> MRGSHHHHHHTDPQGDAAQKTDTSHHDQDHPTFNKITPNLAEFAFSLYRQLAHQSNSTNIFFSPVSIATAFAMLSLGTKADTHDEILEGLNFNLTEIPEAQIHEGFQELLRTLNQPDSQLQLTFGNGLFLSEGLKLVDKFLEDVKKLYHSEAFTVNFGDTEEAKKQINDYVEKGTQGKIVDLVKELDRDTVFALVNYIFFKGKWERPFEVKDTEEEDFHVDQVTTVKVPMMKRLGMFNIQHCKKLSSWVLLMKYLGNATAIFFLPDEGKLQHLENELTHDIITKFLENEDRRSASLHLPKLSITGTYDLKSVLGQLGITKVFSNGADLSGVTEEAPLKLSKAVHKAVLTIDEKGTEAAGAMFLEAIPMSIPPEVKFNKPFVFLMIEQNTKSPLFMGKVVNPTQK

The plasma protein α1-antitrypsin is principally synthesised by hepatocytes and protects lung tissue from degradation by inhibiting neutrophil elastase. It is the archetypal member of the serpin (serine protease inhibitor) superfamily of proteins. In common with other inhibitory serpins, the native fold of α1-antitrypsin is metastable and this property is utilised in the characteristic serpin mechanism of action.

The 2.2 Å crystal structure of Thr114Phe α1-antitrypsin adopts the classic structure of a serpin fold in the native conformation. The polypeptide chain spanning residues 24–393 is highly ordered with the exception of residues 344–351. The root-mean-square deviation (r.m.s.d.) of the mutant and wild-type structures, based on Cα positions, is 0.4 Å. The lack of perturbation elsewhere in the overall structure of Thr114Phe α1-antitrypsin implies that the mutation must be mediating its effect on the fold stability of native α1-antitrypsin from within the cavity flanking β-sheet A. The cavity is well defined in this high-resolution structure, permitting interpretation of the effect of the mutation on cavity filling at the side-chain level. Phe114 makes no interactions with nearby residues, and therefore, its effects are entirely due to partial filling of the cavity and changes in its packing environment during unfolding and polymerisation. The aromatic group of Phe114 closes the upper part of the cavity with its side chain just 3.7 Å from Leu103 and 4.0 Å from Asn104 at the top of helix D, distances that permit favourable van der Waals contacts. The volume partially filling the cavity in Thr114Phe α1-antitrypsin is in a region of high-solvent accessibility in the wild-type protein and also yields the therapeutically desirable combination of effective blockade of polymerisation whilst maintaining inhibitory function. The estimated size of this ideal pharmacophore is 59 Å3, equivalent to 22% of the total cavity volume in wild-type α1-antitrypsin. In order for α1-antitrypsin to adopt either M⁎ conformation, residue 114 must move laterally by 4.6 Å in the plane of β-sheet A. This is limited by local steric clashes in Thr114Phe α1-antitrypsin. The high-resolution structural characterisation of the Thr114Phe mutation presents a more precise pharmacophore target for screening of small fragments capable of mimicking its effects.> GTLTGERPPVFWLQGQGCTGCSVTLLNSVHPSIADVLLKVISLEFHPTVMAWEGEHAIEHMRKVAEKFKGKFFLVIEGSVPVEADGKYCIIGEANHHEISMVDALKEFGPNAAAVLAVGTCAAYGGIPAAEGSETGATAVSKFLGDNGIKTPVVNIPGCPPHPDWIVGTVVLALDAIKKNGLEGGLAEVVKVLDSDGRPTPFFGRNIHENCPYLDKYDEGVMSATFTDKVGCRYDLGCKGPMTMADCFERKWNGGVNWCVQNAVCIGCVEPDFPDGKSPFYQA;> WSHPQFEKGATGRTTIAIDPVTR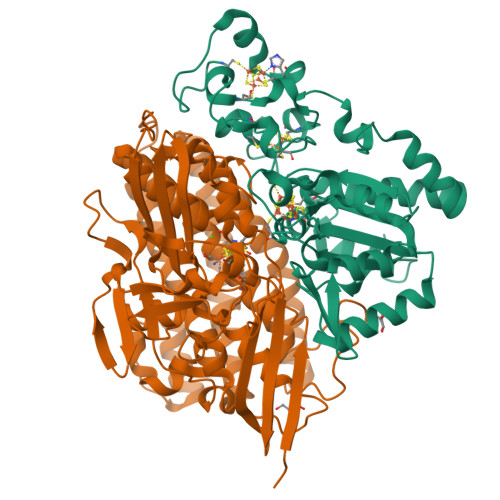IEGHLKAEVVVENGKVVDARLSGGMYRGFETILRGRDPRDASQIVQRICGVCPTAHSTASVLALDEAFGAKVPNNGRITRNLIFGANYLQSHILHFYHLSAQDFVQGPDTAPFVPRFPKSDLRLSKELNKAGVDQYIEALEVRRICHEMVALFGGRMPHVQGQVVGGATEIPTKEKLVEYAARFKKVRDFVEQKYVPVVYTIGSKYKDMFKVGQGFKAALCVGAFPLDNSGKKHLFMPGVYAKGKDMPFDPSKIKEYVKYSWFAEETTGLNYKEGKTIPAPDKAGAYSFVKAPRYDGLSLEVGPLARMWVNNPELSPVGKKLLKDLFGISAKKFRDLGEEAAFSLMGRHVARAEETYYMLGAIEGWLKEIKAGEDTVVMPAVPASAEGTGFTEAPRGSLLHYVKVKDSKIDNYQIVSASLWNCNPRDDMGQRGAVEEALIGIPVDDIQNPVNVARLIRAFDPULSCAVH3-PHENYL-6-(1H-PYRAZOL-4-YL)IMIDAZO[1,2-A]PYRAZINE | C15 H11 N5 | 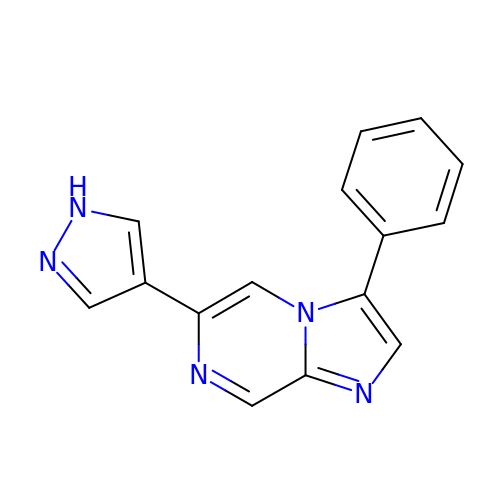YCLNNSSAFUQKBC-UHFFFAOYSA-N>MGHHHHHHAENLYFQGADPFESYNPEFFLYDIFLKFCLKYIDGEICHDLFLLLGKYNILPYDTSNDSIYACTNIKHLDFINPFGVAAGFDKNGVCIDSILKLGFSFIEIGTITPRGQTGNAKPRIFRDVESRSIINSCGFNNMGCDKVTENLILFRKRQEEDKLLSKHIVGVSIGKNKDTVNIVDDLKYCINKIGRYADYIAINVSSPNTPGLRDNQEAGKLKNIILSVKEEIDNLEKNNIMNDEFLWFNTTKKKPLVFVKLAPDLNQEQKKEIADVLLETNIDGMIISNTTTQINDIKSFENKKGGVSGAKLKDISTKFICEMYNYTNKQIPIIASGGIFSGLD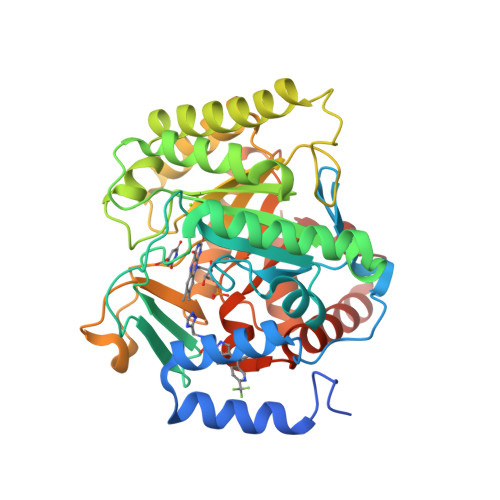ALEKIEAGASVCQLYSCLVFNGMKSAVQIKRELNHLLYQRGYYNLKEAIGRKHSKS[2x]> GPLGSQLIQEFTAAQRRGEIGRMREVAAVLLHFKGYAHCVDVYIKQCQEGAYMRNDVFEDIAILCQRVNKQVGEVFCSPETVMAKLIQSIFENKIQAHVKERLDETRNSDVEQYLKNLYDLYTRTTALAAKLTDYNLGSDKHTFLSKLIKNIFSCYLESYIDMERQYLQNRSGMILQRYYDSKNHQKRPVGTGSITNLPLGPSIDTHGETLLSQEVVVNLLQETRHAFERCNKLSDPADLPKNAFSIFLILVEYLCVDHIDYALEIGLSAIPSADAKNANLYFLDVVQQANTIFHLFDKQFNDHLMPLISSSPKLTECLHKKKEVIEQMEVKLDTGIDRTLNCMIGQMKYILTTEQKKTDFKPEDENNVMIQYTTACSKVCAYVGKQVERVRRSMDGKNVDTVLTELGVRFHRLIHEHLQQFSYSSMGGMLAICDVAEYRRSAKDFRVPLVLQLFDTLHALCNLLVVAPDNLKQVCSGEQLTNLDRNLLHAFVQLRVDYRSARLGRHFS

In the initial step of the fusion, it has been postulated that the vesicles and the plasma membrane are physically and reversibly connected through a heterooctameric protein complex termed the exocyst complex2. The exocyst complex consists of Sec3, Sec5, Sec6, Sec8, Sec10, Sec15, Exo70 and Exo84. Sec10 appears to serve as a central hub for bridging these two assembly modules, possibly through its interaction with Sec6 and/or Sec82324. In this study, we report the near-full-length structure of zebrafish Sec10 (zSec10).

Among the expression constructs tested in this study, we obtained clusters of daggerlike small crystals from zSec10195–708 (Δ385–394). Bromide soaking improved the diffraction from ~4 Å to 3 Å or higher. The structure of zSec10195–708 (Δ385–394) was determined by a single-wavelength anomalous dispersion (SAD) method and refined to 2.73 Å. Residues 378–384 and 395–402 were invisible, probably owing to the structural disorder. The final refined model includes 10 bromide atoms and 2 water molecules. zSec10 folds into an elongated rod with dimensions of 150 Å × 40 Å × 25 Å. The structure of zSec10 can be divided into five domains A–E, each of which is composed of an antiparallel helix bundle. Helix H7 is shared between domains B and C, whereas helix H11 is shared between domains C and D. These two long helices serve as the bridge connecting two adjoining subdomains. In contrast, zSec10 shows no substantial charge polarity on its surface, but several negatively or positively charged pockets were observed in its C-terminal half. The corresponding region of zSec10 forms a cave with negative charges, which are derived primarily from acidic residues on the loop connecting domains C and D. This cave could electrostatically interact with the conserved lysine residues (i.e., Lys3, Lys7 and Lys12) of Arf6 in the N-terminal region, which is required for the interaction with Sec1027.>[4x]MGHHHHHHMEEFTDKVAIVTGGSSGIGLAVVDALVRYGAKVVSVSLDEKSDVNVSDHFKIDVTNEEEVKEAVEKTTKKYGRIDILVNNAGIEQYSPLHLTPTEIWRRIIDVNVNGSYLMAKYTIPVMLAIGHGSIINIASVQSYAATKNAAAYVTSKHALLGLTRSVAIDYAPKIRCNAVCPGTIMTPMVIKAAKMEVGEDENAVERKIEEWGRQHPMGRIGRPEEVAEVVAFLASDRSSFITGACLTV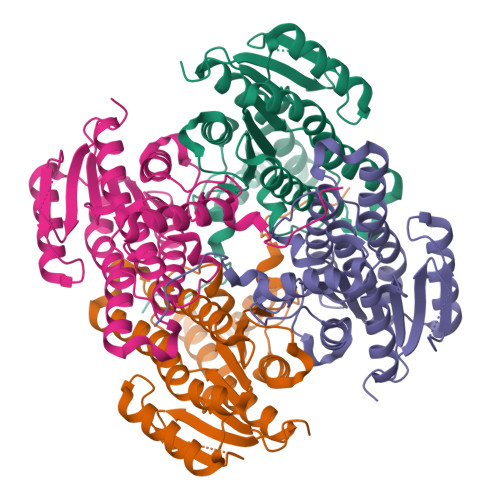DGGLLSKLPISTPNADNSHH> MRQVWFSWIVGLFLCFFNVSSAAQYEPPATWENVDYKRTIDVSNAYISETIEITIKNIASEPATEYFTAFESGIFSKVSFFSAYFTNEATFLNSQLLANSTTAPGDDGESEIRYGIIQFPNAISPQEEVSLVIKSFYNTVGIPYPEHVGMSEEQHLLWETNRLPLSAYDTKKASFTLIGSSSFEEYHPPNDESLLGKANGNSFEFGPWEDIPRFSSNETLAIVYSHNAPLNQVVNLRRDIWLSHWASTIQFEEYYELTNKAAKLSKGFSRLELMKQIQTQNMRQTHFVTVLDMLLPEGATDHYFTDLVGLVSTSHAERDHFFIRPRFPIFGGWNYNFTVGWTNKLSDFLHVSSGSDEKFVASIPILNGPPDTVYDNVELSVFLPEGAEIFDIDSPVPFTNVSIETQKSYFDLNKGHVKLTFSYRNLISQVANGQVLIKYDYPKSSFFKKPLSIACYIFTALMGVFVLKTLNMNVTN;> MAKAPKANTPKVTSTSSAVLTDFQETFKTSKRAYFAQIEKYPKLKLIDTFCFFLVLLGVIQCTFIILIRDNFPFNAFLAGFIICVGQFVLLMSLRLQLCNSFPGISKNRAFAEFIVASLILHFVCLHFIN;> MKWCSTYIIIWLAIIFHKFQKSTATASHNIDDILQLKDDTGVITVTADNYPLLSRGVPGYFNILYITMRGTNSNGMSCQLCHDFEKTYHAVADVIRSQAPQSLNLFFTVDVNEVPQLVKDLKLQNVPHLVVYPPAESNKQSQFEWKTSPFYQYSLVPENAENTLQFGDFLAKILNISITVPQAFNVQEFVYYFVACMVVFIFIKKVILPKVTNKWKLFSMILSLGILLPSITGYKFVEMNAIPFIARDAKNRIMYFSGGSGWQFGIEIFSVSLMYIVMSALSVLLIYVPKISCVSEKMRGLLSSFLACVLFYFFSYFISCYLIKNPGYPIVF;> MISDEQLNSLAITFGIVMMTLIVIYHAVDSTMSPKN;> MTYEQLYKEFHSSKSFQPFIHLDTQPKFAICGLIVTLAVLSSALFAVGSKSSYIKKLFFYTILSVIGSLFAGLTTVFASNSFGVYV;> MGSDRSCVLSVFQTILKLVIFVAIFGAAISSRLFAVIKFESIIHEFDPWFNYRATKYLVNNSFYKFLNWFDDRTWYPLGRVTGGTLYPGLMTTSAFIWHALRNWLGLPIDIRNVCVLFAPLFSGVTAWATYEFTKEIKDASAGLLAAGFIAIVPGYISRSVAGSYDNEAIAITLLMVTFMFWIKAQKTGSIMHATCAALFYFYMVSAWGGYVFITNLIPLHVFLLILMGRYSSKLYSAYTTWYAIGTVASMQIPFVGFLPIRSNDHMAALGVFGLIQIVAFGDFVKGQISTAKFKVIMMVSLFLILVLGVVGLSALTYMGLIAPWTGRFYSLWDTNYAKIHIPIIASVSEHQPVSWPAFFFDTHFLIWLFPAGVFLLFLDLKDEHVFVIAYSVLCSYFAGVMVRLMLTLTPVICVSAAVALSKIFDIYLDFKTSDRKYAIKPAALLAKLIVSGSFIFYLYLFVFHSTWVTRTAYSSPSVVLPSQTPDGKLALIDDFREAYYWLRMNSDEDSKVAAWWDYGYQIGGMADRTTLVDNNTWNNTHIAIVGKAMASPEEKSYEILKEHD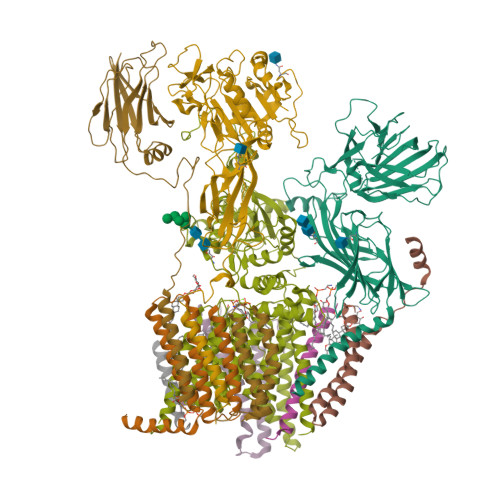VDYVLVIFGGLIGFGGDDINKFLWMIRISEGIWPEEIKERDFYTAEGEYRVDARASETMRNSLLYKMSYKDFPQLFNGGQATDRVRQQMITPLDVPPLDYFDEVFTSENWMVRIYQLKKDDAQGRTLRDVGELTRSSTKTRRSIKRPELGLRV;> MRTDWNFFFCILLQAIFVVGTQTSRTLVLYDQSTEPLEEYSVYLKDLEQRNYKLEYLDINSTSTTVDLYDKEQRLFDNIIVFPTKGGKNLARQIPVKQLIKFFENEGNILCMSSPGAVPNTIRLFLNELGIYPSPKGHVIRDYFSPSSEELVVSSNHLLNKYVYNARKSEDFVFGESSAALLENREQIVPILNAPRTSFTESKGKCNSWTSGSQGFLVVGFQNLNNARLVWIGSSDFLKNKNQDSNQEFAKELLKWTFNEKSVIKSVHAVHSHADGTSYDEEPYKIKDKVIYSVGFSEWNGEEWLPHIADDIQFELRQVDPYYRLTLSPSGNDSETQYYTTGEFILPDRHGVFTFLTDYRKIGLSFTTDKDVKAIRHLANDEYPRSWEISNSWVYISAICGVIVAWIFFVVSFVTTSSVGKKLETFKKTN;> MQFFKTLAALVSCISFVLAYVAQDVHVSFPSTAGKSRVMIGKVEPRIGIDETVPTTITVEDPNEVIQVNFAIESTNKPFQNTLLIGLPNKNLEMAFEPEIKDNGKLSMYKYRIDLAKLDAALLQEASRSPEPIKATLILASSTAKPKENLFREILQLNLNFDVDHSDSSLVDKFGIKPEIHHIFHAEPKRVAKPIAVIFVLIIFITILSLIVTWLNSCAAAFNNIPTGVTAVYFLGFIATIVGFEVIFARYYLGTSIFETLFSSLYLGAPGLLTSTKFLRSFGQTI>MVDRGPLLTSAIIFYLAIGAAIFEVLEEPHWKEAKKN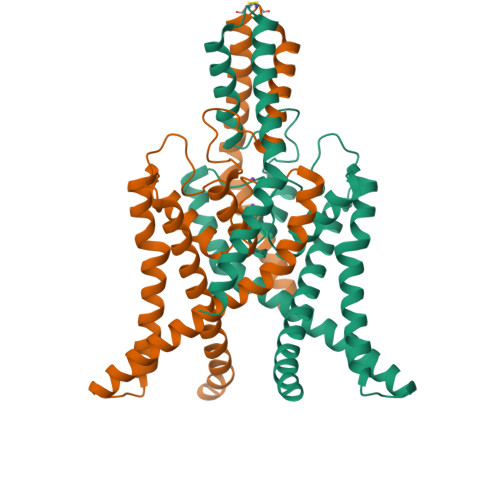YYTQKLHLLKEFPCLSQEGLDKILQVVSDAADQGVAITGNQTFNNWNWPNAMIFAATVITTIGYGNVAPKTPAGRLFCVFYGLFGVPLCLTWISALGKFFGGRAKRLGQFLTRRGVSLRKAQITCTAIFIVWGVLVHLVIPPFVFMVTEEWNYIEGLYYSFITISTIGFGDFVAGVNPSANYHALYRYFVELWIYLGLAWLSLFVNWKVSMFVEVHKAIKKRRRRRKESFESSPHSRKALQMAGSTASKDVNIFSFLSKKEETYNDLIKQIGKKAMKTSGGGERVPGPGHGLGPQGDRSNSLEVLFQ[2x]> MNCRSEVLEVSVEGRQVEEAMLAVLHTVLLHRSTGKFHYAAAGTYSIGTVGTQDVDCDFIDFTYVRVSSEELDRALRKVVGEFKDALRNSGGDGLGQMSLEFYQKKKSRWPFSDECIPWEVWTVKVHVVALATEQERQICREKVGEKLCEKIINIVEVMNRHEYLPKMPTQSEVDNVFDTGLRDVQPYLYKISFQITDALGTSV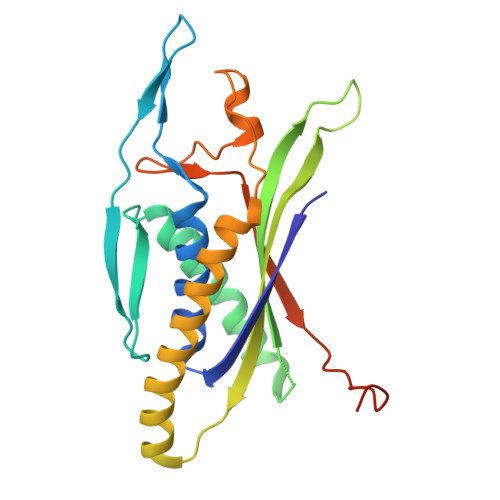TTTMRRLIKDTLAL>[2x]GVALHRPDVYLLP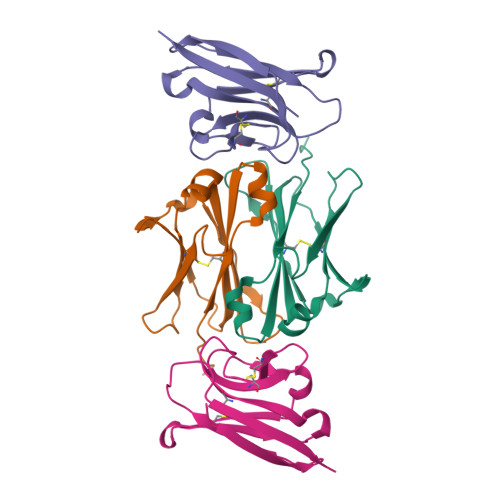PAREQLNLRESATITCLVTGFSPADVFVQWMQRGQPLSPEKYVTSAPMPEPQAPGRYFAHSILTVSEEEWNTGETYTCVVAHEALPNRVTERTVDKSTG;>RILPEVKVEGELGGSVTIKCPLPEMHVRIYLCREMAGSGTCGTVVSTTNFIKAEYKGRVTLKQYPRKNLFLVEVTQLTESDSGVYACGAGMNTDRGKTQKVTLNVHS[2x]>[4x]MSEVEFSHEYWMR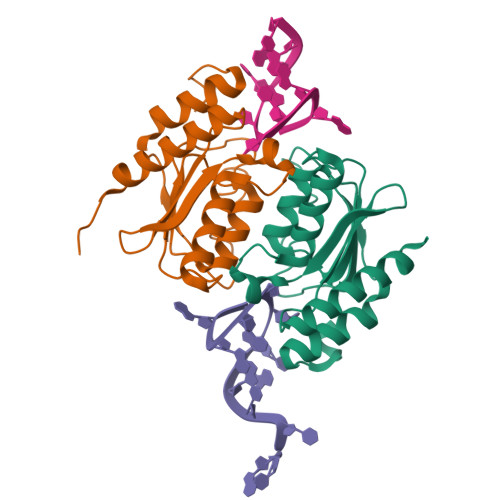HALTLAKRARDEREVPVGAVLVLNNRVIGEGWNRAIGLHDPTAHAEIMALRQGGLVMQNYRLYDATLYSTFEPCVMCAGAMIHSRIGRVVFGVRNAKTGAAGSLMDVLHHPGMNHRVEITEGILADECAALLCRFFRMPRRVFNAQKKAQSSTD> DYMPMS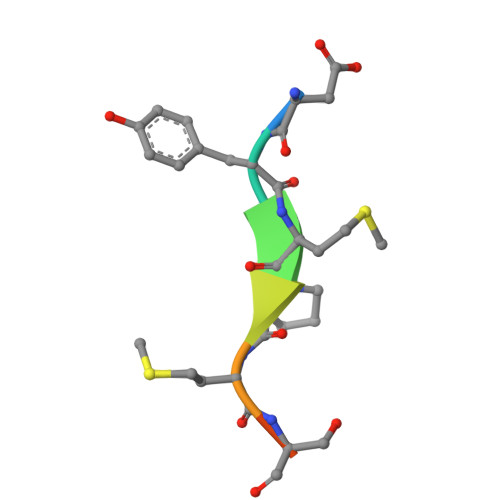PK>[3x]PTSDDIFEREYKYGAHNYHPLPVALERGKGIYLWDVEGRKYFDFLSSYSAVNQGHCHPKIVNALKSQVDKLTLTSRAFYNNVLGEYEEYITKLFNYHKVLPMNTGVEAGETACKLARKWGY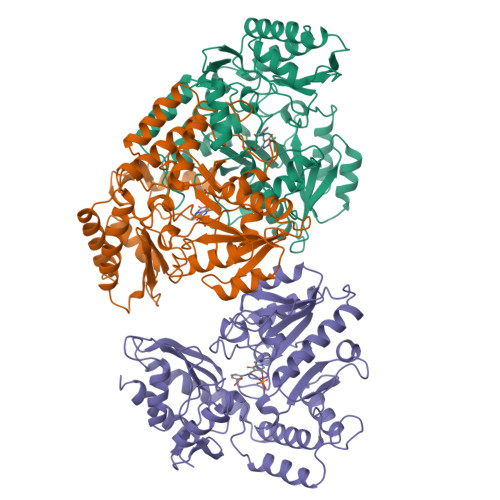TVKGIQKYKAKIVFAAGNFWGRTLSAISSSTDPTSYDGFGPFMPGFDIIPYNDLPALERALQDPNVAAFMVEPIQGEAGVVVPDPGYLMGVRELCTRHQVLFIADEIQTGLARTGRWLAVDYENVRPDIVLLGKALSGGLYPVSAVLCDDDIMLTIKPGEHGSTYGGNPLGCRVAIAALEVLEEENLAENADKLGIILRNELMKLPSDVVTAVRGKGLLNAIVIKETKDWDAWKVCLRLRDNGLLAKPTHGDIIRFAPPLVIKEDELRESIEIINKTILSF>[4x]MDTMRQRILVVDDDASLAEMLTIVLRGEGFDTAVIGDGTQALTAVRELRPDLVLLDLMLPGMNGIDVCRVLRADSGVPIVMLTAKTDTVDVVLGLESG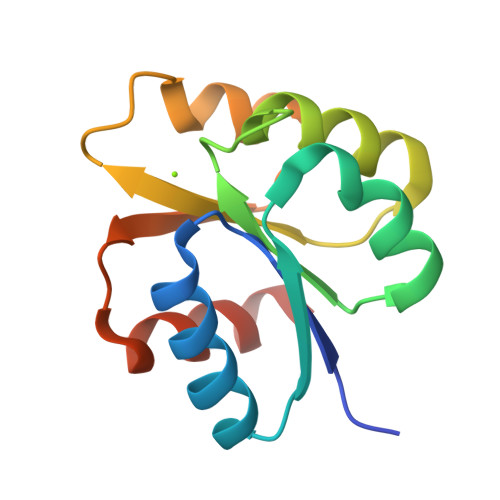ADDYIMKPFKPKELVARVRARLRRNDD> IIPVEEENPDFWNREAAEALGAAKKLQPAQTAAKNLIIFLGDGMGVSTVTAARILKGQKKDKLGPEIPLAMDRFPYVALSKTYNVDKHVPDSGATATAYLCGVKGNFQTIGLSAAARFNQCNTTRGNEVISVMNRAKKAGKSVGVVTTTRVQHASPAGTYAHTVNRNWYSDADVPASARQEGCQDIATQLISNMDIDVILGGGRKYMFRMGTPDPEYPDDYSQGGTRLDGKNLVQEWLAKRQGARYVWNRTELMQASLDPSVTHLMGLFEPGDMKYEIHRDSTLDPSLMEMTEAALRLLSRNPRGFFLFVEGGRIDHGHHESRAYRALTETIMFDDAIERAGQLTSEEDTLSLVTADHSHVFSFGGYPLRGSSIFGLAPGKARDRKAYTVLLYGNGPGYVLKDGARPDVTESESGSPEY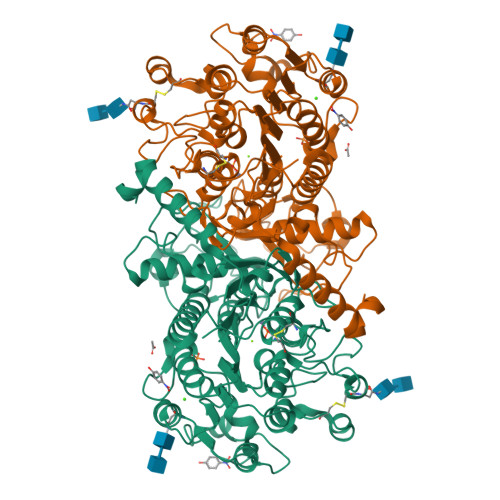RQQSAVPLDEETHAGEDVAVFARGPQAHLVHGVQEQTFIAHVMAFAACLEPYTACDLAPPAGTTD>[2x]MVDRGPLLTSAIIFY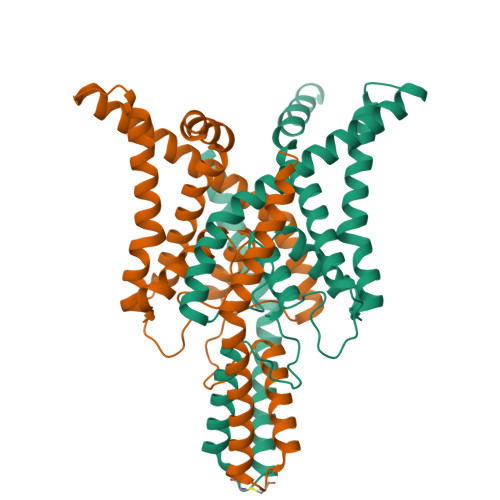LAIGAAIFEVLEEPHWKEAKKNYYTQKLHLLKEFPCLSQEGLDKILQVVSDAADQGVAITGNQTFNNWNWPNAMIFAATVITTIGYGNVAPKTPAGRLFCVFYGLFGVPLCLTWISALGKFFGGRAKRLGQFLTRRGVSLRKAQITCTAIFIVWGVLVHLVIPPFVFMVTEEWNYIEGLYYSFITISTIGFGDFVAGVNPSANYHALYRYFVELWIYLGLAWLSLFVNWKVSMFVEVHKAIKKRRRRRKESFESSPHSRKALQMAGSTASKDVNIFSFLSKKEETYNDLIKQIGKKAMKTSGGGERVPGPGHGLGPQGDRSNSLEVLF We analysed a multidomain xylanase (Xyl) from the hindgut metagenome of the snouted harvester termite Trinervitermes trinervoides that releases xylobiose and xylotriose from beech and birch xylan and wheat arabinoxylan. The four domains of Xyl include an N-terminal GH11 xylanase domain, two family 36-like carbohydrate-binding domains CBM36-1 and 2, and a C-terminal CE4 esterase domain. Instead, individual domains and domain combinations were investigated structurally and for possible interdomain interactions. Xyl exemplifies a “beads-on-a-string” protein where the individual domains are “beads” each connected by a linker (string), with each domain retaining its individual function- making the synthesis of novel super enzymes for rapid and efficient degradation of bio-waste to biofuels within reach.

Crystals were obtained using 10 mg/mL Xyl-GH11 in 50 mM Na acetate pH 4.8, 500 mM (NH4)2SO4 at 18°C. Diffraction data were collected on beamline ID29 (ESRF, Grenoble, France) and processed using XDS. The Xyl-GH11 domain crystallised in space group P1 diffracting X-rays to a resolution of 1.39 Å but yielding a low completeness of only 87.5 or 67.0% for the entire data set or the shell of highest resolution. This is a result of the low symmetry space group and a non-ideal crystal orientation, yet still reveals most critical structural details. Two symmetrically independent Xyl-GH11 domains occupy the asymmetric unit. Each Xyl-GH11 adopts a β-jelly-roll fold composed of 14 β-strands, one α-helix and mostly short loops of up to five residues. The domain resembles a partially closed right hand with the β-sheets forming palm and fingers while an extended loop between β-strands 8 and 9 forms the thumb. The substrate-binding cleft of Xyl-GH11 lies within the inner β-sheet cleft. Comparing Xyl-GH11 to related enzymes including the Trichoderma reesei enzyme Xyn11 (TrXyn11), identify Glu122 and Glu212 as catalytic nucleophile and general acid, respectively. The latter adopts “up” and “down” conformations as part of its catalytic cycle.

>[2x]ATTLYENKTGTEDGYDYELWKDSGNTSMILNGGGTFSCQWSNINNCLFRKGKKFGGNQSYQQIGNISFDYGCDYHPNGNSYLCVYGWTTSPLVEFYIVDSWGSWRPPGGSPKGQIYVDGGTYDVYETTRVNQPSIQGNTTFQQYFSVRTERRTSGTINVTEHFKAWERMGMRMGNIYEAALNVEGYQSSGSANVYKNNMTIG> QDNTRKIIIKNFDIPKSVRPNDEVTAVLAVQTELKECMVVKTYLISSIPLQGAFNYKYTACLCDDNPKTFYWDFYTNRTVQIAAVVDVIRELGICPDDAAVI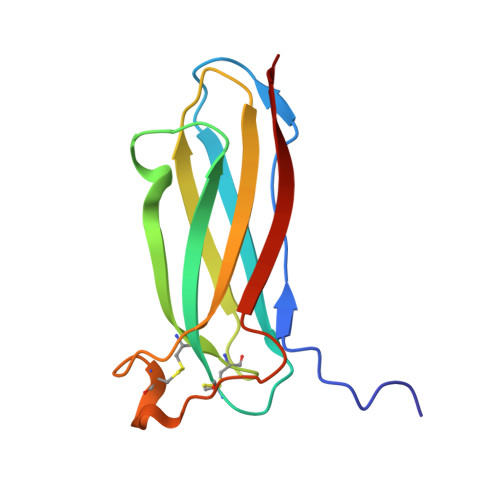PIKNNRFYTIEILKVE> IGMAPGGYVAPKAVWLPAVKAKGLEISGTFTHRQGHIYMEMNFTNKALQHMTDFAIQFNKNSFGVIPSTPLAIHTPLMPNQSIDVSLPLNTLGPVMKMEPLNNLQVAVKNNIDVFYFSCLIPLNVLFVEDGKMERQVFLATWKDIPNENELQFQIKECHLNADTVSSKLQNNNVYTIAKRNVEGQDMLYQSLKLTNGIWILAELRIQPGNPNYTLSLKCRAPEVSQYIYQVYDSILKN;>[2x]DDDIVFEDFARQRLKGMKDD

Adaptor protein complex 2 α and β-appendage domains act as hubs for the assembly of accessory protein networks involved in clathrin-coated vesicle formation. The C-terminal “appendage domains” of the large subunits recruit interaction partners from the cytosol facilitating their concentration at sites of coated pit formation. We identify a large repertoire of β-appendage interactors by mass spectrometry. These interact with two distinct ligand interaction sites on the β-appendage (the “top” and “side” sites) that bind motifs distinct from those previously identified on the α-appendage. We solved the structure of the β-appendage with a peptide from the accessory protein Eps15 bound to the side site and with a peptide from the accessory cargo adaptor β-arrestin bound to the top site.

To understand the specificity of the β-appendage top site we solved the crystal structure of β2-appendage in combination with β-arrestin P-long. By circular dichroism this peptide, in solution, is not helical (unpublished data) but in our β-appendage crystal structure the β-arrestin peptide is folded as an α-helix in a groove between α-helix 1 and the antiparallel β-sheet of the platform sub-domain. Thus the peptide folds on appendage binding. In our structure of the β-appendage:β-arrestin P-long co-complex, residues D3–R13 were clearly visible and the induced helix breaks down after the arginine residue. The main interacting residues on the helix are D3xxF6xxF9xxxR13. Our density for D3 is not well defined but the side-chain appears to make hydrogen bonds with R834 and R879. F6 is in a hydrophobic environment created by F837, L838, and I876. F9 projects into a hydrophobic space lined by W841 and Y888. The guanidino group of R13 forms hydrogen bonds with E849 and E902. The core motif, as revealed by the structure, is DxxFxxFxxxR, with the additional constraint that this must be found in the context of an α-helix, unlike the unfolded nature of peptide interactions known for other appendages.>GSRDNLLFGDEIITNGFHSCESDEEDRASHASSSDWTPRPRIGPY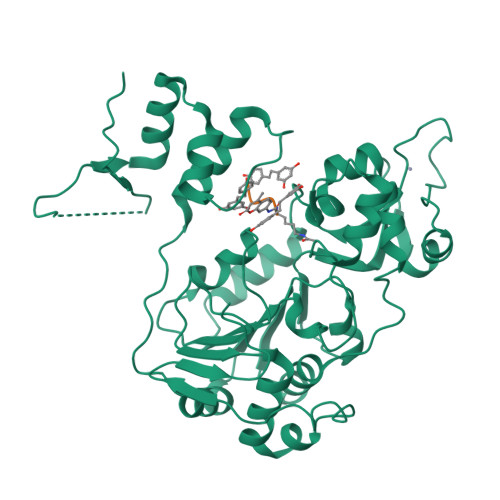TFVQQHLMIGTDPRTILKDLLPETIPPPELDDMTLWQIVINILSEPPKRKKRKDINTIEDAVKLLQESKKIIVLTGAGVSVSSGIPDFRSRDGIYARLAVDFPDLPDPQAMFDIEYFRKDPRPFFKFAKEIYPGQFQPSLCHKFIALSDKEGKLLRNYTQNIDTLEQVAGIQRIIQCHGSFATASCLICKYKVDCEAVRGDIFNQVVPRCPRCPADEPLAIMKPEIVFFGENLPEQFHRAMKYDKDEVDLLIVIGSSLKVRPVALIPSSIPHEVPQILINREPLPHLHFDVELLGDCDVIINELCHRLGGEYAKLSSNPVKLSEITEQYLFLPPNRYIFHGAEVYSDSEDDV[3x]>SGSGSTAEPDLKTALKAVIPAKRELFKQVKERSDEVIGEVKVANVIGGMRGLKSMLWEGSVLDPEEGIRFHGKTIKDCQKELPKGTSGTEMLPEAMFWLLLTGQVPSTNQVRAFSRELAEQSHLPQHILDLIKSFPRSMHPMTQLSIAVAALNTESKFAKAYEKGLSKADYWEPTFDDSISLLAKIPRVAALVFRPDEVDQVGTQALDASQDWSYNFAELLGKGGKENQDFHDLLRLYLALHGDHEGGNVSAHATHLVGSALSDPFLSYSAGLLG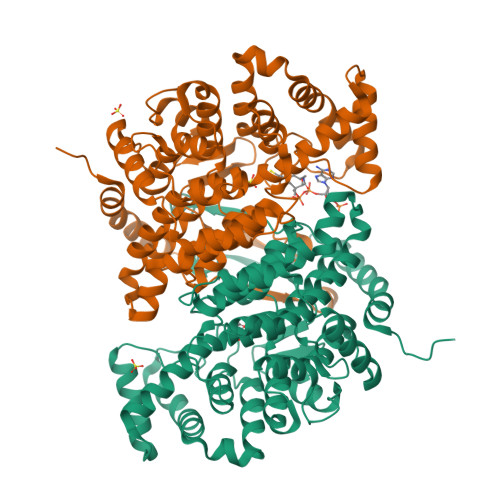LAGPLHGLAAQEVLRWILAMQDKIGTKFTDDDVRNYLWDTLKSGRVVPGYGHAVLRKPDPRFQALMDFAATRPDVLANPVFQLVKKNSEIAPAVLTEHGKTKNPHPNVDAASGVLFYHYGFQQPLYYTVTFGVSRALGPLVQLIWDRALGLPIERPKSINLLGLKK[2x]> MAEEHEKGVPMVLAPQMGAIDATVESIRYRAQLIARNQKLDSG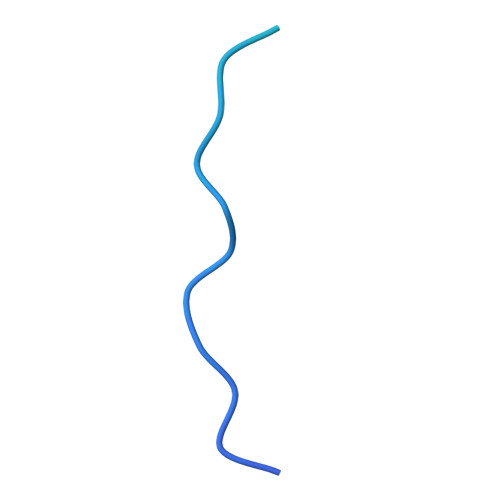VAATGIIGFAAGFLFSLLMVIVLPVAVGL> GAMADSELVAQWEKVQIKTFTKWVNMHLAKKGRKINDVTTDFKNGVELCALLEIIGETTIKCVTNPKMRIQMTENLDKALRFIQSRDVKLTGIGPTDIVDGNVKLTLGLVWTLILRFAISELSAEGLSAKQGLLLWCQKKCEPYPVKVENFSESFKDGKVFCALIHRHRPDLLDWETVGEDDRANLEKAFDVAEKELGIPKLLDVDDIVNMPRPDERSVMTYVAALYKVFSSNDQVEKAGKRAGNFLDLLRATEGMVHDYEQRAQALKENIEAAINKMNGVEPSDEYHQVKEQI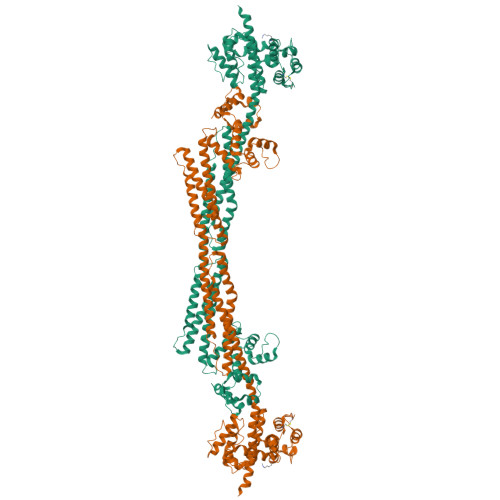NETKNYRKGDKRAFIKEQGDLATLFGQINSKLRGMKRPVYVAPEGLDPKSLEGYIANISEAERALRSKLNTAMRNCLIALRKAFADPANATDAKINEYRTFVTDETSEAPLEEQVATLKAKLEELKQVEAQLPPIEEAEKACGDANIEDNEYTDVSFDDLQFNYEQTVSMFEKKIVYIEAQINEASSGVTAEQMQEFKQSFDAFNGGHNGILDKLEFRSCLSSMGLIDIDFTGGEDAQYDAIYNNVTKGENGVSFDNYVQYMKEKNDENPSPEQLNEIFSTIAAGKDSITETDMQKAGMSAEQIEYVKANLPQKGDGYDYAAWVKTN> EQQRFPQRYIELAIVVDHGMYTKYSSNFKKIRKRVHQMVSNINEMCRPLNIAITLALLDVWSEKDFITVQADAPTTAGLFGDWRERVLLKKKNHDHAQLLTDTNFARNTIGWAYVGRMCDEKYSVAVVKDHSSKVFM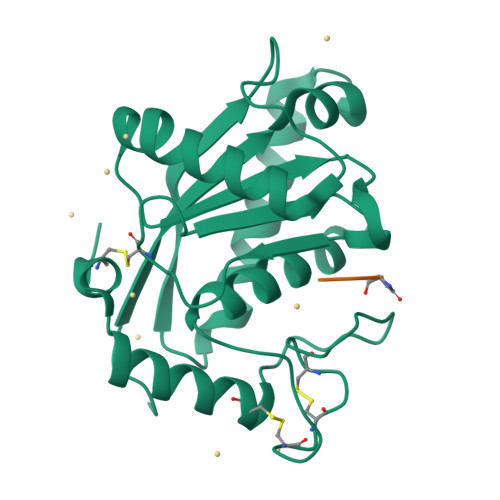VAVTMTHELGHNLGMEHDDKDKCKCTTCIMSAVISDKQSKLFSDCSKDYYQTFLTNDNPQCILNAP;> QNW>MHDANIRVAIAGAGGRMGRQLIQAALALEGVQLGAALEREGSSLLGSDAGELAGAGKTGVTVQSSLDAVKDDFDVFIDFTRPEGTLNHLAFCRQHGKGMVIGTT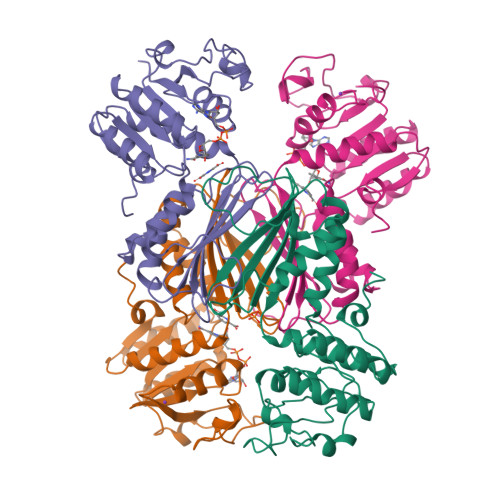GFDEAGKQAIRDAAADIAIVFAANFSVGVNVMLKLLEKAAKVMGDYTDIEIIEAHHRHKVDAPSGTALAMGEAIAHALDKDLKDCAVYSREGHTGERVPGTIGFATVRAGDIVGEHTAMFADIGERLEITHKASSRMTFANGAVRSALWLSGKESGLFDMRDVLDLNNL[4x]>EEIRPKEVYLDRKLLTLEDKELGSGNFGTVKKGYYQMKKVVKTVAVKILKNEANDPALKDELLAEANVMQQLDNPYIVRMIGICEAESWMLVMEMAELGPLNKYLQQNRHVKDKNIIELVHQVSMGMKYLEESNFVHRDLAARNVLLVTQHYAKISDFGLSKALRADENYYKAQTHGKWPVKWYAPECINYYKFSSKSDVWSFGVLMWEAFSYGQKPYRGMKGSEVTAMLEKGERMGCPAGCPREMYDLMNLCWTYDVENRPGFAAVEL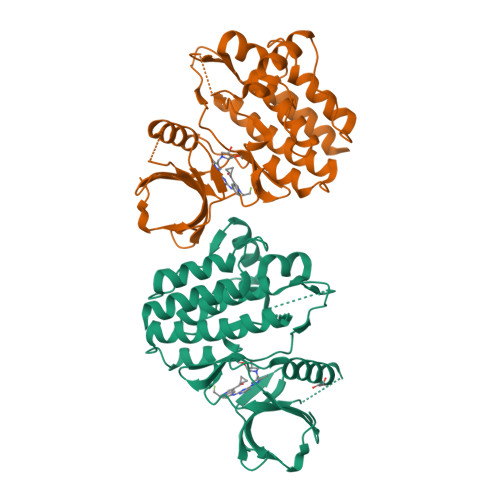RLRNYYYDVVNLEHHHHHHHH[2x]>[4x]VTPTKPINLVVLPVQNDGSTGLHWANLQKRTPLMQVPVLVDLNGNHLWVNCEQQYSSKTYQAPFCHSTQCSRANTHQCLSCPAASRPGCHKNTCGLMSTNPITQQTGLGELGEDVLAIHATQGSTQQLGPLVTVPQFLFSCAPSFLVQK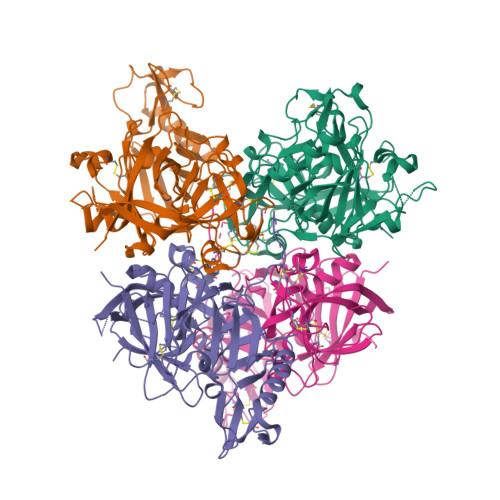GLPRNTQGVAGLGHAPISLPNQLASHFGLQRQFTTCLSRYPTSKGAIIFGDAPNNMRQFQNQDIFHDLAFTPLTITLQGEYNVRVNSIRINQHSVFPLNKISSTIVGSTSGGTMISTSTPHMVLQQSVYQAFTQVFAQQLPKQAQVKSVAPFGLCFNSNKINAYPSVDLVMDKPNGPVWRISGEDLMVQAQPGVTCLGVMNGGMQPRAEITLGARQLEENLVVFDLARSRVGFSTSSLHSHGVKCADLFNFANA>[2x]MGSITENTSWNK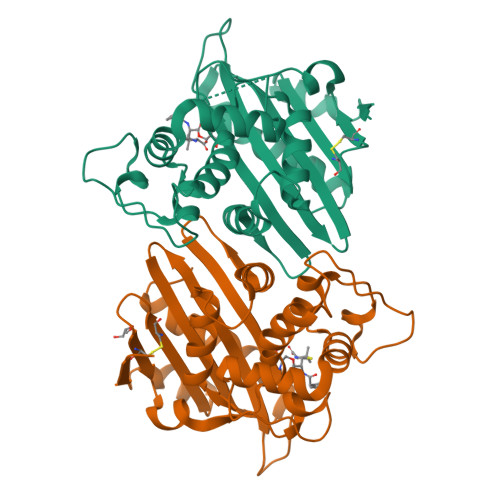EFSAEAVNGVFVLCKSSSKSCATNDLARASKEYLPASTFKIPNAIIGLETGVIKNEHQVFKWDGKPRAMKQWERDLTLRGAIQVSAVPVFQQIAREVGEVRMQKYLKKFSYGNQNISGGIDKFALEGQLRISAVNQVEFLESLYLNKLSASKENQLIVKEALVTEAAPEYLVHSKTGFSGVGTESNPGVAWWVGWVEKETEVYFFAFNMDIDNESKLPLRKSIPTKIMESEGIIGG> MMLSATQPLSEKLPAHGCRHVAIIMAGNGRWAKKQGKIRAFGHKAGAKSVRRAVSFAANNGIEALTLYAFSSENWNRPAQEVSALMELFVWALDSEVKSLHRHNVRLRIIGDTSRFNSRLQERIRKSEALTAGNTGLTLNIAANYGGRWDIVQGVRQLAEKVQQGNLQPDQIDEEMLNQHVCMHELA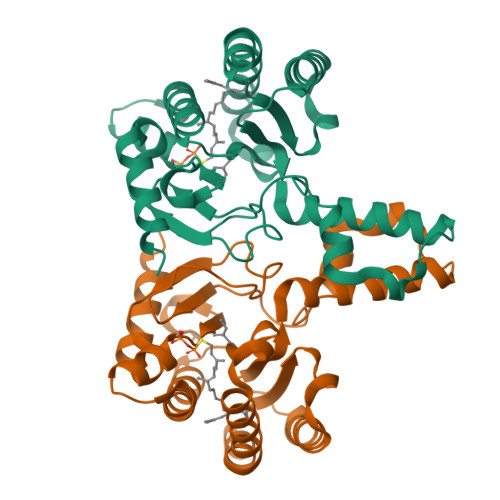PVDLVIRTGGEHRISNFLLWQIAYAELYFTDVLWPDFDEQDFEGALNAFANRERRFGGTEPGDETA> LPPP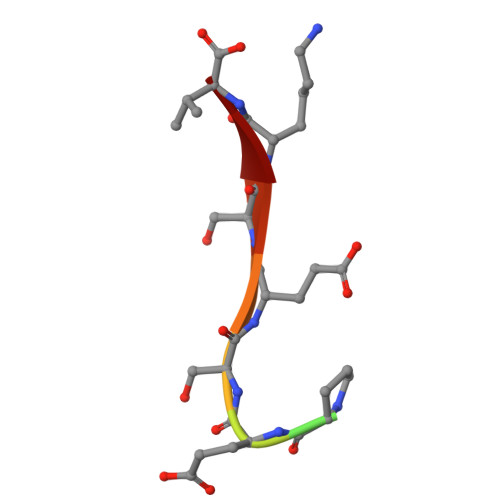ESESKV> MENTENSVDSKSIKNLEPKIIHGSESMDSGISLDNSYKMDYPEMGLCIIINNKNFHKSTGMTSRSGTDVDAANLRETFRNL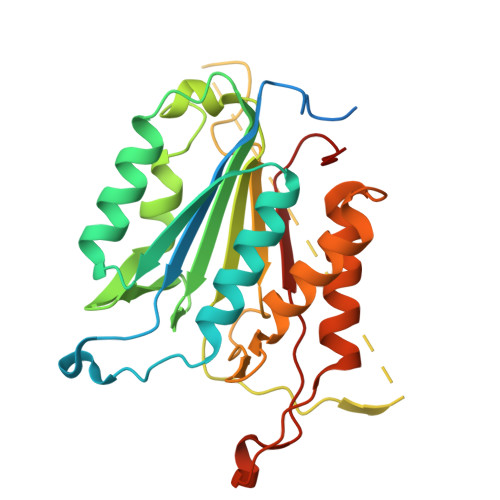KYEVRNKNDLTREEIVELMRDVSKEDHSKRSSFVCVLLSHGEAGIIFGTNGPVDLKKITNFFRGDRCRSLTGKPKLFIIQACRGTELDCGIETDSGVDDDMACHKIPVEADFLYACSTAPGYYSWRNSKDGSWFIQSLCAMLKQYADKLEFMHILTRVNRKVATEFESFSFDATFHAKKQIPCIVSMLTKELYFYH> MRHYKTLRYYETVFAVKPTLSEEEMKKKFEQVKEFIKQKGG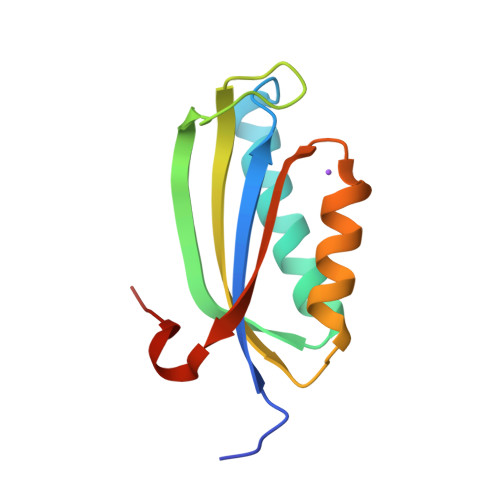EILYEEDWGMRQLAYPIQKFNNARYFLVQFKTENPQLPNELDFQLKIDEDVIRWLNIQIKESEVKKNAQ>MKRRDILKGGLAAGALALLPRGHTQGALQNQPSLGRRYRNLIVFVYDGFSWEDYAIAQAYARRRQGRVLALERLLARYPNGLINTYSLTSYVTESSAAGNAFSCGVKTVNGGLAIHADGTPLKPFFAAAKEAGKAVGLVTTTTVTHATPASFVISNPDRNAEERIAEQYLEFGAEVYLGGGDRFFNPARRKDGKDLYAAFAAKGYGVVRTPEELVRSNATRLLGVFADGHVPYEIDRRFQGLGVPSLKEMVQAALPRLAAHRGGFVLQVEAGRIDHANHLNDAGATLWDVLAADEVLELLTAFVDRNPDTLLIVVSDHATGVGGLYGAGRSYLESSQGVDLLEPQRASFEHMLRVLGQAPEASQVKEAFRAMKGVDLEDAEAERVVRAIREKVYWPEGVRQGVQPANTMAWAMVQRDAQKPDRPNIGWSSGQHTASPVMLLLYGQGLRFVNLGLVDNTHVFRLMGEALGLRYQNPVMSEEEALEILKARPQGMR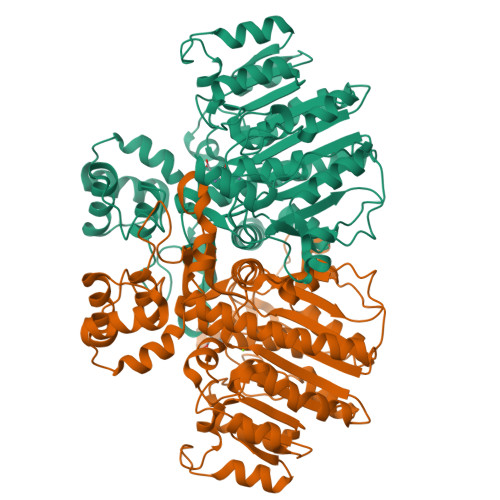HPEDVWA[2x]>KEISNTVSNEMSKKASYDNVDTLIEKGRYNTKYNYLKRMEKYYPNAMAYFDKVTINPQGNDFYINNPKVELDGEPSMNYLEDVYVGKALLTNDTQQEQKLKSQSFTCKNTDTVTATTTHTVGTSIQATAKFTVPFNETGVSLTTSYSFANTNTNTNSKEITHNVPSQDILVPANTTVEVIAYLKKVNVKGNVKLVGQVSGSEWGEIPSYLAFPRDGYKFSLSDTVNKSDLN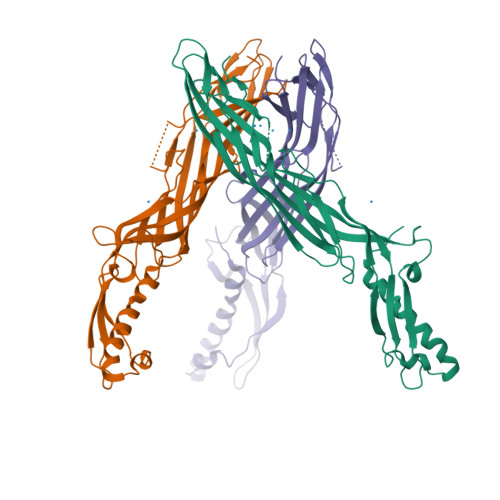EDGTININGKGNYSAVMGDELIVKVRNLNTNNVQEYVIPVDKKEKSNDSNIVKYRSLSIKAPGIK[3x]>GSSGSSGMQIGKIIKVSGPLVMAENMSEASIQDMCLVGDLGVIGEIIEMRQDVASIQVYEETSGIGPGEPVRSTGEALSVELGPGIISQMFDGIQRPLDTFMEVTQSNFLGRGVQLPALDHEKQWWFEATIEEGTEVSAGDIIGYVDETKIIQHKIMVPNGIKGTVQKIESGSFTIDDPICVIETEQGLKELTMMQKWPVRRGRPIKQKLNPDVPMITGQRVIDTFFPVTKGGAAAVPGPFGAGKTVVQHQIAKWSDVDLVVYVGCGERGNEMTDVVNEFPELIDPNTGESLMERTVLIANTSNMPVAAREASIYTGITIAEYFRDMGYDVAIMADSTSRWAEALREMSGRLEEMPGDEGYPAYLGSRLAEYYERSGRVIALGSDQREGSITAISAVSPSGGDISEPVTQNTLRVVKVFWGLDSSLAQKRHFPSINWIQSYSLYSTEVGRYMDQILQQDWSDMVTEGMRILQEEEQLNEIVRLVGIDSLSDNDRLTLEVAKSIREDYLQQNAFDDVDTFTSREKQFNMLKVILTFGKEARKALSLGAYFNEIMEGTVAVRERISRSKYIPEEELAKISSINEEIKETIQLIVSEGGMTDD[3x];>GSSGSSGMIKEYRTIKEVVGPLMAVEKVSGVKYEELIEVRMQNGEIRRGQVLEVQEDKAMVQIFEGTSGINLKNSSVRFLGHPLQLGVSEDMIGRVFDGLGRPKDNGPEILPEKYLDINGEVINPIARDYPDEFIQTGISAIDHLNTLVRGQKLPVFSGSGLPHKELAAQIARQATVLDSSDDFAVVFAAIGITFEEAEFFMEDFRQTGAIDRSVMFMNLANDPAIERIATPRMALTAAEYLAYEKGMHVLVIMTDMTNYAEALREISAARREVPGRRGYPGYLYTNLATLFERAGRIRGLKGSVTQIPILTMPEDDKTHPIPDLTGYITEGQIILTRELYKSGIQPPIDVLPSLSRLKDKGTGAGKTREDHAATMNQLFAAYAQGKQAKELAVVLGESALSDIDKIYAKFAERFENEYVNQGFYTNRTITETLDLGWELLAMLPRTELKRIKDDLLDKYLPEGK[3x];> GSSGSSGMRLNVNPTRMELTRLKKQLTTATRGHKLLKDKQDELMRQFILLIRKNNELRQAIEKETQTAMKDFVLAKSTVEEAFIDELLALPAENVSISVVEKNIMSVKVPLMNFQYDETLNETPLEYGYLHSNAELDRSIDGFTQLLPKLLKLAEVEKTCQLMAEEIEKTRRRVNALEYMTIPQLEETIYYIKMKLEENERAEVTRLIKVKNMGTEE;> MTYKIGVVGDKDSVSPFRLFGFDVQHGTTKTEIRKTIDEMAKNEYGVIYITEQCANLVPETIERYK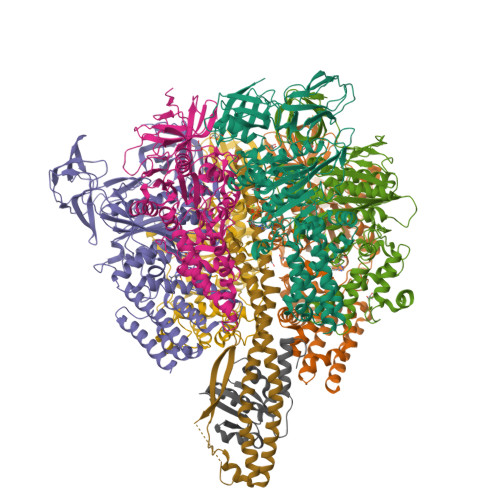GQLTPAIILIPSHQGTLGIGLEEIQNSVEKAVGQNILSGPSSGENLYFQ> GMADPGPDPESESESVFPREVGLFADSYSEKSQFCFCGHVLTITQNFGSRLGVAARVWDAALSLCNYFESQNVDFRGKKVIELGAGTGIVGILAALQGGDVTITDLPLALEQIQGNVQANVPAGGQAQVRALSWGIDHHVFPANYDLVLGADIVYLEPTFPLLLGTLQHLCRPHGTIYLASKMRKEHGTESFFQHLLPQHFQLELAQRDEDENVNI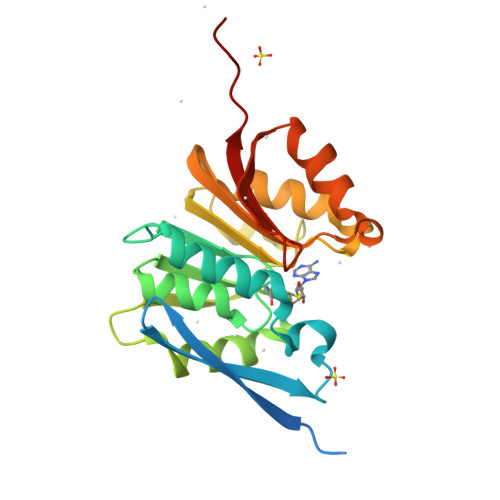YRARHREPRPA>GAMVVHEPVDMTEVIDRSLERVRRRRSDIEFEVTVTPWQVIGDSSGLGRAVLNVLDNAAKWSPPGGRVGVRLYQIDPGHAELVITDQGPGIPPQERHLVFERFFRSASARSMPGSGLGLAIVKQVVLKHGGALRVDYADPAAQ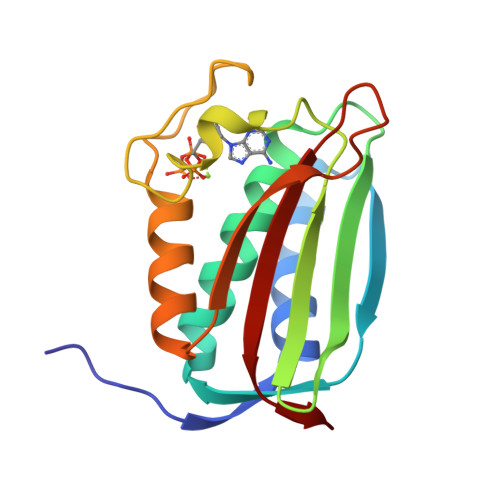PPGTAIHIVLPGRPM[4x]> IKGGLFADIASHPWQAAIFAKHRRSPGERFLCGGILISSCWILSAAHCFQERFPPHHLTVILGRTYRVVPGEEEQKFEVEKYIVHKEFDDDTYDNDIALLQLKSDSSRCAQESSVVRTVALPPADLQLPDWTECELSG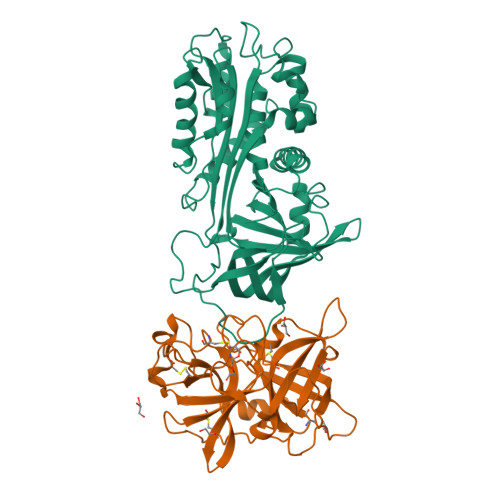YGKHEALSPFYSERLKEAHVRLYPSSRCTSQHLLQRTVTDNMLCAGDTRSGGPQANLHDACQGDAGGPLVCLNDGRMTLVGIISWGLGCGQKDVPGVYTKVTNYLDWIRDNMRP;> VHHPPSYVAHLASDFGVRVFQQVAQASKDRNVVFSPYGVASVLAMLQLTTGGETQQQIQAAMGFKIDDKGMAPALRHLYKELMGPWNKDEISTTDAIFVQRDLKLVQGFMPHFFRLFRSTVKQVDFSEVERARFIINDWVKTHTKGMISHLLGTGAVDQLTRLVLVNALYFNGQWKTPFPDSSTHRRLFHKSDGSTVSVPMMAQTNKFNYTEFTTPDGHYYDILELPYHGDTLSMFIAAPYEKEVPLSALTNILSAQLISHWKGNMTRLPRLLVLPKFSLETEVDLRKPLENLGMTDMFRQFQADFTSLSDQEPLHVALALQKVKIEVNESGTVASSSTAVIVSARMAPEEIIIDRPFLFVVRHNPTGTVLFMGQVMEP> SELDPKGQHVCVASSPSAELQCCAGWRQKDQECTIPICEGPDACQKDEVCVKP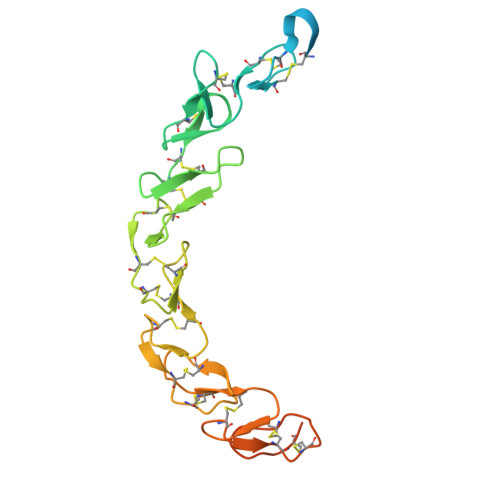GLCRCKPGFFGAHCSSRCPGQYWGPDCRESCPCHPHGQCEPATGACQCQADRWGARCEFPCACGPHGRCDPATGVCHCEPGWWSSTCRRPCQCNTAAARCEQATGACVCKPGWWGRRCSFRCNCHGSPCEQDSGRCACRPGWWGPECQQSRHHHHHH>[8x]MSTIAITNVTLIDGLGGLPRPATTVIVEGDRFATVGPSDSTPVPEGATVVDGNRRWMVPGYVNGNVHLLDAWMFMAGPGTIEYLAR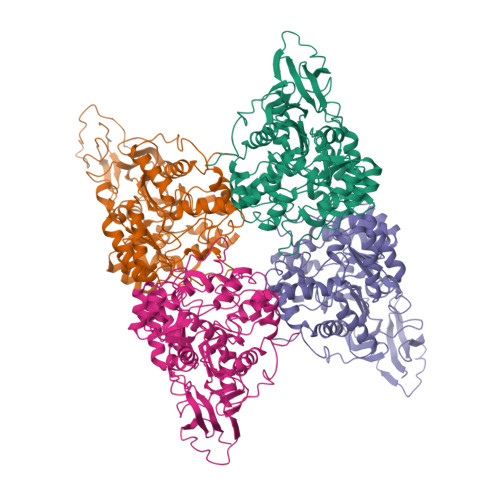WEGRYVEVIEEAAQLALRNGVTTVFDTHNAIEPVLAARDRINAGISQGARIFAAGTIVGMGGPFSADFHFAGRTAATRTFVDRIDSMFEAGVGHQLSLLPRKEVRARVRDYLSRGVDMLKIAVSDHIVFTLVDRSVGFDRSYQTFSRPVLEVMVEEARAAGVPVLTHSVSVEALDTSVELGADVLIHANYTLGQEIPNYLIDKIVASDSWAGLQTVHDQHRQGLEDVGSWAAALAGEPYATNERNLISANAKILLNTDAGCPSKDHLADLSPVEREDRPWTIGNDHFHWTQSMVEKGMSPLEAISAATINVARAYGKADQIGSVETGKLADFVLLDQDPVDDIRNLRSITEVFQAGAAVDRAALPTTPLVTAHPA>[2x]GKKMMTTDGNTATAHVAYAMSEVAAIYPITPSSTMGEEADDWAAQGRKNIFGQTLTIREMQSEAGAAGAVHGALAAGALTTTFTASQGLLLMIPNMYKISGELLPGVFHVTARAIAAHALSIFGDHQDIYAARQTGFAMLASSSVQ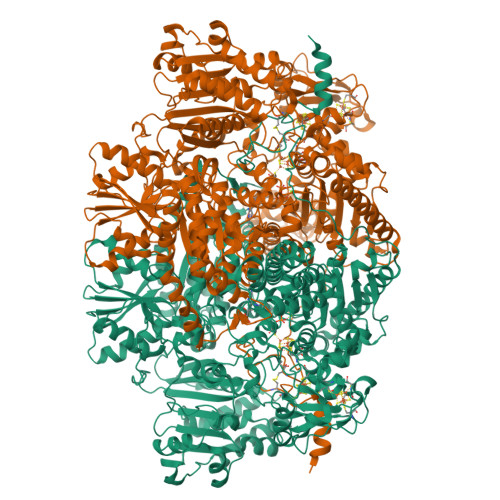EAHDMALVAHLAAIESNVPFMHFFDGFRTSHEIQKIEVLDYADMASLVNQKALAEFRAKSMNPEHPHVRGTAQNPDIYFQGREAANPYYLKVPGIVAEYMQKVASLTGRSYKLFDYVGAPDAERVIVSMGSSCETIEEVINHLAAKGEKIGLIKVRLYRPFVSEAFFAALPASAKVITVLDRTKEPGAPGDPLYLDVCSAFVERGEAMPKILAGRYGLGSKEFSPAMVKSVYDNMSGAKKNHFTVGIEDDVTGTSLPVDNAFADTTPKGTIQCQFWGLGADGTVGANKQAIKIIGDNTDLFAQGYFSYDSKKSGGITISHLRFGEKPIQSTYLVNRADYVACHNPAYVGIYDILEGIKDGGTFVLNSPWSSLEDMDKHLPSGIKRTIANKKLKFYNIDAVKIATDVGLGGRINMIMQTAFFKLAGVLPFEKAVDLLKKSIHKAYGKKGEKIVKMNTDAVDQAVTSLQEFKYPDSWKDAPAETKAEPMTNEFFKNVVKPILTQQGDKLPVSAFEADGRFPLGTSQFEKRGVAINVPQWVPENCIQCNQCAFVCPHSAILPVLAKEEELVGAPANFTALEAKGKELKGYKFRIQINTLDCMGCGNCADICPPKEKALVMQPLDTQRDAQVPNLEYAARIPVKSEVLPRDSLKGSQFQEPLMEFSGACSGCGETPYVRVITQLFGERMFIANATGCSSIWGASAPSMPYKTNRLGQGPAWGNSLFEDAAEYGFGMNMSMFARRTHLADLAAKALESDASGDVKEALQGWLAGKNDPIKSKEYGDKLKKLLAGQKDGLLGQIAAMSDLYTKKSVWIFGGDGWAYDIGYGGLDHVLASGEDVNVFVMDTEVYSNTGGQSSKATPTGAVAKFAAAGKRTGKKDLARMVMTYGYVYVATVSMGYSKQQFLKVLKEAESFPGPSLVIAYATCINQGLRKGMGKSQDVMNTAVKSGYWPLFRYDPRLAAQGKNPFQLDSKAPDGSVEEFLMAQNRFAVLDRSFPEDAKRLRAQVAHELDVRFKELEHMAATNIFESFAPAGGKADGSVDFGEGAEFCTRDDTPMMARPDSGEACDQNRAGTSEQQGDLSKRTKK Bdellovibrio bacteriovorus is a bacterium that preys upon a wide range of other Gram-negative bacteria, entering their periplasm and consuming them from within. Proteomic and structural analyses of vesicle contents reveal several fibre-like proteins, which we name the mosaic adhesive trimer (MAT) superfamily, and show localization on the predator surface before prey encounter. Structural studies reveal a variety of domain usages (and therefore binding capabilities) at the fibre C-termini, placing these on intertwined trimeric β-prisms. Using independent but complementary approaches, we identified and characterized a MAT superfamily of trimeric fibre proteins with diverse adhesive tips, able to fulfil the long-sought-after role of multiplicity of molecular recognition and handling of diverse epitopes (across a wide prey range), by the bacterial predator B. bacteriovorus.

We next characterized two more divergent NS74s, Bd2439 and Bd2734, obtaining a tip-only variant of Bd2734 (residues T691–L843, 1.8 Å) and a longer construct of Bd2439 (G837–D1107, 1.6 Å). Bd2439 is modular, formed by a β-helix N850–V968, a R969 linker that coordinates the carboxy terminus and a compact β-domain tip from S970–D1107. Mapping a sequence alignment to Bd2439 identifies a conserved interfacial pocket (Y1031, R1040, E1044, H1053 and H1055 from one monomer; R1022 and Y1097 from another). Thermal unfolding experiments confirm this specificity, revealing a biphasic unfolding whose second phase is shifted in the presence of sugars that contain these features. Bd2439 showed strong binding to Proteus mirabilis OXK glycan, with weaker (but significant) binding to glycans from E. coli K-235 and Serratia marcescens. Our demonstration of a MAT binding pocket capable of recognizing two adjacent hydroxyls presumably explains part of this specificity, but the ubiquity of this feature in surface glycans and relative specificity of Bd2439 suggest that multiple flanking pockets will provide additional selectivity. The fact that none of the single-gene-deletion mutants were significantly defective in predation on Proteus mirabilis hints that there are multiple factors and several MAT proteins involved, but our GlcNAc-bound Bd2439 structure identifies a potential motif that may be used (in part) to select for saccharides in Proteus mirabilis and Proteus mirabilis-like glycans.

>[3x]MDIGINSDPHHHHHHGGLDIVNNATGDDNRDDLNIRTYGATETSSLIMLRARGTASAPAAVQTGDRLGGVLFRGWNGTAWMGSGQILSVAEENFTTAVKTNLQFHVGGAGEAMRISNTGNVGIGTTTTTEKLNVQGNVAVSGEITSVRSWGIKRGPTSFSANYINVWNSGYHVGSSIDCTTSTTGCRILKAGTYEIRCVQRAGTSGNSVYVGIALNGDRTALESRNDVLWNHSHTAYSGSYTESNFMGTLSANDLITCGAPVNTMAADLVYAVPAYNGTMQIKRVD> GSHMLVKTISRTIESESGFLQPTLDVIATLPADDRSKKIPISLVVGFKQEASLNSSSSLSCYYYAIPLMRDRHINLKSGGSNVVGIPLLDTKDDRIRDMARHMATIISERFNRPCYVTWSSLPSEDPSMLVANHLYILKKCLDLLKTELGE;> MISYEFQTHLPKGKDSSLNASSENKELYVQATHFNNTILLQIRLNGEMDSTYEVSSKGLNPILDINVPLAGNLGNTGGDYDDEEEEFVRDHLSDYQVVTKLGDSADPKVPVV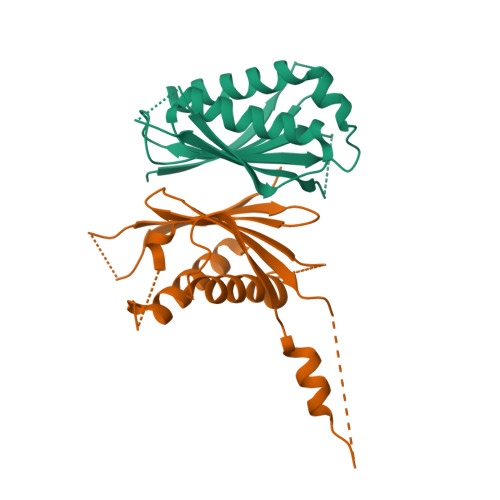CVQIAELYRRVILPEVSGTMAQDNMQFSLLISMSSKIWRATKEQSADDNDFGKLVFVLKCIKDMYAK> MLTKVIAQAHIDHFTKWFERADKIVIVSHVSPDGDAIGSSLGLYHFLDSQDKIVNVIVPNAFPDFLKWMPGSKDILLYDRYQEFADKLIMEADVICCLDFNALKRIDEMSDIVAASPGRKIMIDHHLYPEDFCRITISHPEISSTSELVFRLICRMGYFSDISKEGAECIYTGMMTDTGGFTYNSNNREIYFIISELLSKGIDKDDIYRKVYNTYSESRLRLMGYVLSNMKVYKDYNSALISLTKEEQGKFDYIKGDSEGFVNIPLSIKNVCFSCFL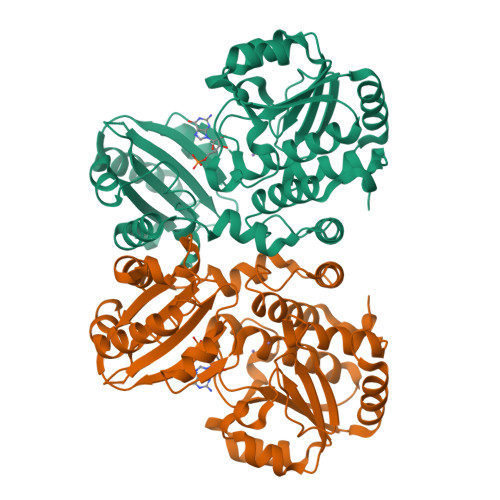REDTEKKMIKISLRSVGKFPCNRLAAEFFNGGGHLNASGGEFYGTMEEAVKVFEQALEKYKPLLKELEHHHHHH>[10x]SMDFDFLKNLSLEEL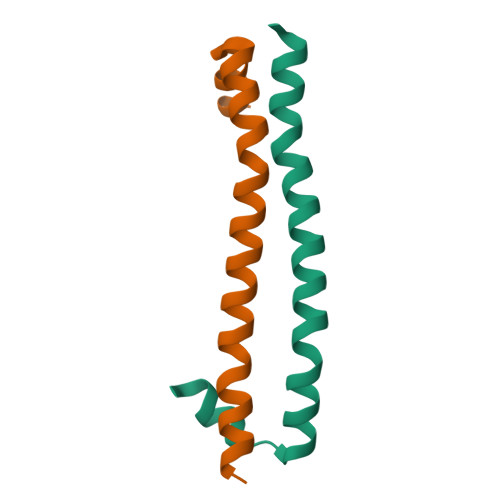QMRLKALDPMMEREIEELRQRYTAKRQPILDAMDAK> ADDYATTRYPIVLVHGLTGTDKYAGVLEYWYGIQEDLQQHGATVYVANLSGFQSDDGPNGRGEQLLAYVKTVLAATGATKVNLVGHSQGGLTSRYVAAVAPDLVASVTTI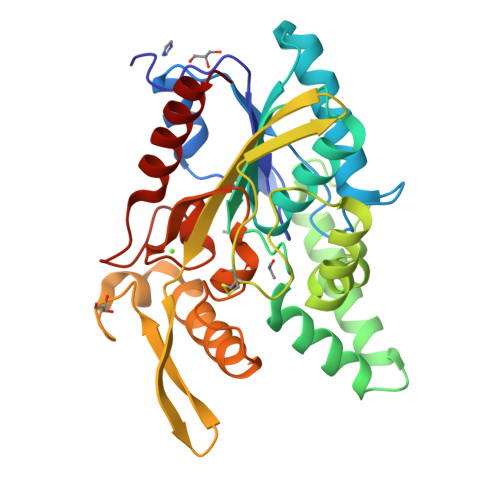GTPHRGSEFADFVQGVLAYDPTGLSSSVIAAFVNVFGILTSSSHNTNQDALASLKTLTTAQAATYNQNYPSAGLGAPGSCQTGAPTETVGGNTHLLYSWAGTAIQPTLSVFGVTGATDTSTIPLVDPANALDPSTLALFGTGTVMINRGSGQNDGLVSKCSALYGQVLSTSYKWNHIDEINQLLGVRGAFAEDPVAVIRTHANRLKLAGV>[6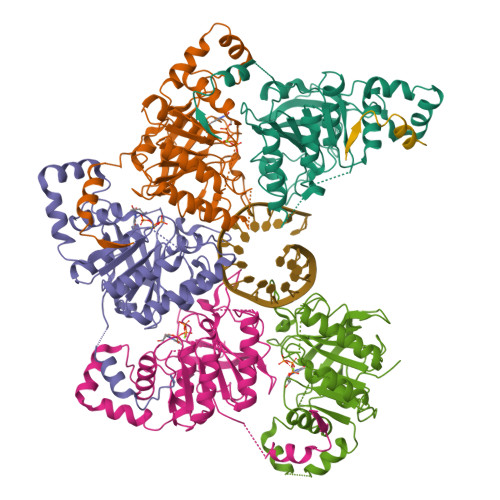x]MDNSHDSDSVFLYHIPCDNCGSSDGNSLFSDGHTFCYVCEKWTAGNEDTKERASKRKPSGGKPMTYNVWNFGESNGRYSALTARGISKETCQKAGYWIAKVDGVMYQVADYRDQNGNIVSQKVRDKDKNFKTTGSHKSDALFGKHLWNGGKKIVVTEGEIDMLTVMELQDCKYPVVSLGHGASAAKKTCAANYEYFDQFEQIILMFDMDEAGRKAVEEAAQVLPAGKVRVAVLPCKDANECHLNGHDREIMEQVWNAGPWIPDGVVSALSLRERIREHLSSEESVGLLFSGCTGINDKTLGARGGEVIMVTSGSGMGKSTFVRQQALQWGTAMGKKVGLAMLQESVEETAEDLIGLHNRVRLRQSDSLKREIIENGKFDQWFDELFGNDTFHLYDSFAEAETDRLLAKLAYMRSGLGCDVIILDHISIVVSASGESDERKMIDNLMTKLKGFAKSTGVVLVVICHLKNPDKGKAHEEGRPVSITDLRGSGALRQLSDTIIALERNQQGDMPNLVLVRILKCRFTGDTGIAGYMEYNKETGWLEPSSYSGEEESHSESTDWSNDTDF> WVPHELTENQKNRRFEVSSSLILRNHNEPFLDRIVTCDEKWILYDNRRRSAQWLDQEEAPKHFPKPILHPKKVMVTIWWSAAGLIHYSFLNPGETITSEKYAQEIDEMNQKLQRLQLALVNRKGPILLHDNARPHVAQPTLQKLNELGYEVLPHPPYSPDLLPTNY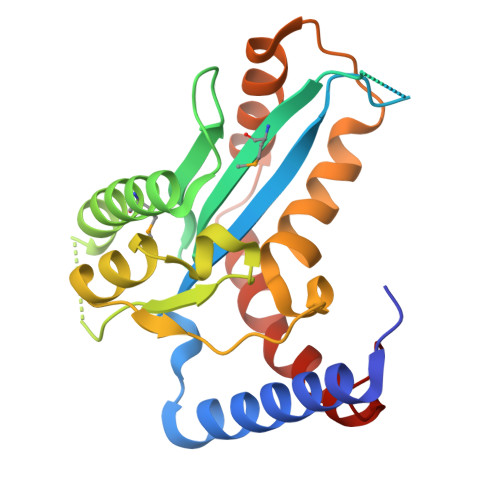HVFKHLNNFLQGKRFHNQQDAENAFQEFVESQSTDFYATGINQLISRWQKCVDCNGSYFD> GHMASGSMSLATILREGTSEEHKAAESSAFIRSFMKGILEKGTYARHLEAFYYVYESMEEELERNKNNLVLKSIYFPELYRKNALLEDLQFFYGTWKP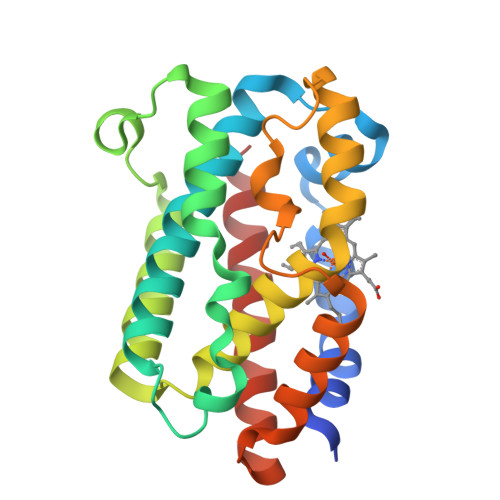NDHQPSVATQDYVQRIRKISETQPELLAAHSYVRYLGDLSGGQILKKVAARALNLPEGKGISFYEFPMIQDINGFKQNYRTALDSLPVNDSEKQSILAESKQVFLLNQGIFSEL> MNRSFVSSADLRGLTAAFCGSLTCQKRFWAKPK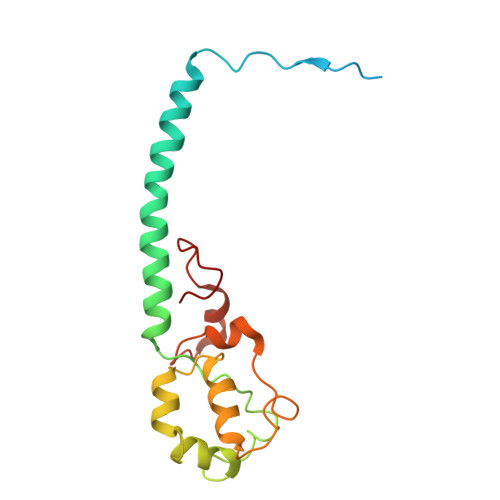KRPKVGPGFHEKAQKWRDEYLLDRHRVLADSLRAYVDFSSTKRVEPWDTRFAPFDRVEKDGVYILTRYLMDDKLQLCNYHHRPVKRMLCNVGLMGPQVTTTARWKPYRFATNPANTTRAERTFTKDKTVFTGYHHD> AKDEDK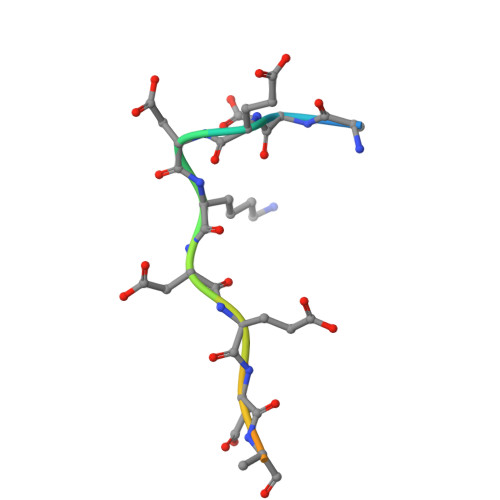DEDEKEKAA>GGGGSMSTAEPAPDPTNPSTSGLAPTTNGIGSPPPTASAATKFSILTKFLRRKNQVHTTTAQQNEFMQKYMPNGNSNAVQPAATGGQPASSDGGSAIEVPPPKESYAVRIRKYLANYTQDPSTDNFYYWTCVVTVAYIYNLLFVIARQVFNDLIGPSSQSLCRFYNGTLNSTTQVECTYNMLTNMKEMPTYSQYPDLGWSKYWHFRMLWVFFDLLMDCVYLIDTFLNYRMGYMDQGLVVREAEKVTKAYWQSKQYRIDGISLIPLDYILGWPIPYINWRGLPILRLNRLIRYKRVRNCLERTETRSSMPNAFRVVVVVWYIVIIIHWNACLYFWISEWIGLGTDAWVYGHLNKQSLPDDITDTLLRRYVYSFYWSTLILTTIGEVPSPVRNIEYAFVTLDLMCGVLIFATIVGNVGSMISNMSAAWTEFQNKMDGIKQYMELRKVSKQLEIRVIKWFDYLWTNKQSLSDQQVLKVLPDKLQAEIAMQVHFETLRKVRIFQDCEAGLLAELVLKLQLQVFSPGDFICKKGDIGREMYIVKRGRLQVVDDDGKKVFVTLQEGSVFGELSILNIAGSKNGNRRTANVRSVGYTDLFVLSKTDLWNALREYPDARKLLLAKGREILKKDNLLDENAPEEQKTVEEIAEHLNNAVKVLQTRMARLIVEHSSTEGKLMKRIEMLEKHLSRYKALARRQKTMHGVSIDGGDISTDGVDERVRPPRLRQTKTIDLPTGTESESLLK[4x]

CNG channels open when bound with cGMP and conduct Na+ and Ca2+ ions into photoreceptor cells. The gating ring transmits cGMP binding/unbinding-triggered conformational changes in the CNBD to the TMD, where a cavity gate formed by two hydrophobic residues in S6 opens and closes. Cryo-EM structures of the Caenorhabditis elegans TAX-4 CNG channel carrying the analogous mutation, R421W, show that most apo channels are open. R421W disrupts this interaction, destabilizes the closed state, and stabilizes the open state.

Given that the R421W mutation appears to greatly attenuate cGMP activation of TAX-4, we at first hypothesized that either TAX-4_R421W could not bind cGMP or cGMP-bound TAX-4_R421W would be closed due to mutation-induced defective coupling of cGMP binding and gate opening. To our surprise, cGMP-bound TAX-4_R421W is open and its structure (determined at 2.9 Å resolution with C4 symmetry) is identical to the previously reported structure of cGMP-bound WT TAX-425. Comparison of mutant and WT channel structures shows an r.m.s.d. of 0.62 Å when all visible amino acids are included. The hydrophobic cavity gate formed by F403 and V407 of S6 opens to the same extent in the mutant channel as in the WT channel, and the CNBD and gating ring in both channels have the same ligand-bound conformation. These results suggest that the R421W mutation does not markedly affect the process of cGMP activation of TAX-4.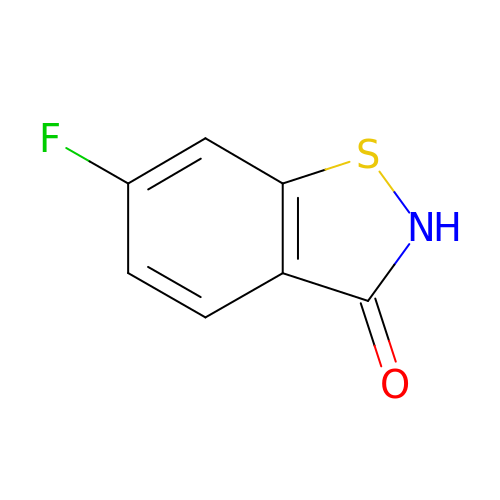6-fluoranyl-1,2-benzothiazol-3-one | C7 H4 F N O S | WLQRIPHXCTXOQC-UHFFFAOYSA-N As the main entry gate of mitochondria, the TOM complex is responsible for transferring ~90% of mitochondrial proteins from the cytosol into the mitochondria. Mitochondrial proteins are primarily synthesized within the cytosolic ribosome and subsequently transferred to specific mitochondrial compartments through the corresponding translocase complexes, including the translocase of the outer mitochondrial membrane (TOM) and the translocase of the inner mitochondrial membrane (TIM23). The TOM complex consisted of two Tom40 pores, which were surrounded by two copies of three small Tom subunits and tethered by two Tom22 molecules. To investigate the transfer process of preproteins from cytosol to the mitochondrial matrix, we captured the TOM–TIM23 supercomplex by translocating Jac1sfGFP to isolated yeast mitochondria to obtain TOM–TIM23–Jac1sfGFP supercomplex.

After the TOM–TIM23–Jac1sfGFP supercomplex was purified from a 100-L culture of Saccharomyces cerevisiae, we further obtained a density map (overall resolution of 4.4 Å) of this supercomplex through cryo-electronic microscopy (cryo-EM) analysis. In the architecture of the TOM–TIM23–Jac1sfGFP supercomplex, the structural features of the TOM complex were significantly clearer than those of the TIM23 complex. Further analysis revealed that the local resolution of the TOM complex structure ranged from 3.0 Å to 6.0 Å. The densities corresponding to Jac1 polypeptides and sfGFP were observed within the Tom40 channel and on the cytosolic side of the Tom40, respectively. The rough densities of the Jac1 polypeptides were mainly distributed close to the cytosolic side of β-strands 10–12 within Tom40 channel, and the remaining densities along β-strands 3–10. Moreover, structural analysis of the Jac1sfGFP-engaged TOM complex revealed two preproteins proximity sites (PPS) on the mitochondrial surface. The PPS1 corresponded to the N-terminus of Tom5 (residues 1–26), while the PPS2 encompassed the loop between β-strands 14 and 15 of Tom40. The PPS1 and PPS2 were situated on the cytosolic side of the TOM complex, potentially functioning in recognizing the incoming preproteins. The PPS1 was close to the β-strands 9–11 of the Tom40. Superposition analysis of the free TOM complex and Jac1sfGFP-engaged TOM complex showed that Tom5 exhibited an ~3-Å movement towards the Tom40 channel in the Jac1sfGFP-engaged TOM complex, suggesting that the Tom5 might respond to the incoming substrates.

>[2x]MSAPTPLAEASQIPTIPALSPLTAKQSKGNFFSSNPISSFVVDTYKQLHSHRQSLELVNPGTVENLNKEVSRDVFLSQYFFTGLRADLNKAFSMNPAFQTSHTFSIGSQALPKYAFSALFANDNLFAQGNIDNDLSVSGRLNYGWDKKNISKVNLQISDGQPTMCQLEQDYQASDFSVNVKTLNPSFSEKGEFTGVAVASFLQSVTPQLALGLETLYSRTDGSAPGDAGVSYLTRYVSKKQDWIFSGQLQANGALIASLWRKVAQNVEAGIETTLQAGMVPITDPLMGTPIGIQPTVEGSTTIGAKYEYRQSVYRGTLDSNGKVACFLERKVLPTLSVLFCGEIDHFKNDTKIGCGLQFETAGNQELLMLQQGLDADGNPLQALPQL;>MVELTEIKDDVVQLDEPQFSRNQAIVEEKASATNNDVVDDEDDSDSDFEDEFDENETLLDRIVALKDIVPPGKRQTISNFFGFTSSFVRNAFTKSGNLAWTLTTTALLLGVPLSLSILAEQQLIEMEKTFDLQSDANNILAQGEKDAAATAN[2x];>MFGLPQQEVSEEEKRAHQEQTEKTLKQAAYVAAFLWVSPMIWHLVKKQWK[2x];>[2x]MDGMFAMPGAAAGAASPQQPKSRFQAFKESPLYTIALNGAFFVAGVAFIQSPLMDMLAPQL;>[2x]MSFLPSFILSDESKERISKILTLTHNVAHYGWIPFVLYLGWAHTSNRPNFLNLLSPLPSV> MATQNVDSGHEDMVHDAQFDYYGKFLATCSSDKMIKIFDVGGENPQHLVDLRGHEGPVWQVAWAHPKFGKILASASYDRKVIVWKEVGNNSWSIIHQYAGHELSVNSISWAPHEFGLSLACASSDGSVTIHNYNNNVWEAPQKIQVSQIGVNSVSWSPAAIPTSLVNSANTIIPAPIKRIVTGSCDNLIKIFKNVEDKWILDKQLEDHKDWVRDVAWAPNIGLPYSKIASCSQDRSVIVWTQDENGVWSGKPLPKFDDIVWRVSWSVIGN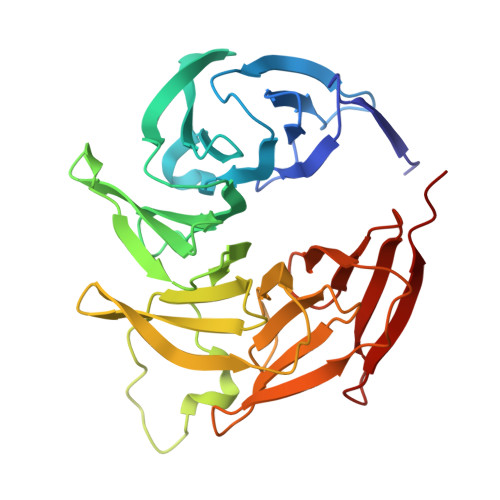ILAVSCGDNQVTLWKEGVDSEWKLISHVENN> MNYNNKILVSESGLSQKHLIHGDEELFQHELKTIFARNWLFLTHDSLIPAPGDYVTAKMGIDEVIVSRQNDGSIRAFLNVCRHRGKTLVSVEAGNAKGFVCSYHGWGFGSNGELQSVPFEKDLYGESLNKKCLGLKEVARVESFHGFIYGCFDQEAPPLMDYLGDAAWYLEPMFKHSGGLELVGPPGKVVIKANWKAPAENFVGDAYHVGWTHASSLRSGESIFSSLAGNAALPPEGAGLQMTSKYGSGMGVLWDGYSGVHSADLVPELMAFGGAKQERLNKEIGDVRARIYRSHLNCTVFPNNSMLTCSGVFKVWNPIDANTTEVWTYAIVEKDMPEDLKRRLADSVQRTVGPAGFWESDDNDNMETASQNGKKYQSRDSDLLSNLGFGEDVYGDAVYPGVVGKSAIGETSYRGFYRAYQAHVSSSNWAEFEHASSTWHTELTKTTDR;> MMINIQEDKLVSAHDAEEILRFFNCHDSALQQEATTLLTQEAHLLDIQAYRAWLEHCVGSEVQYQVISRELRAASERRYKLNEAMNVYNENFQQLKVRVEHQLDPQNWGNSPKLRFTRFITNVQAAMDVNDKELLHIRSNVILH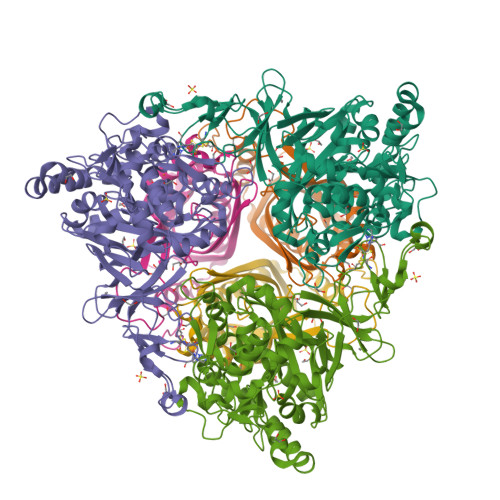RARRGNQVDVFYAAREDKWKRGEGGVRKLVQRFVDYPERILQTHNLMVFL> IESIIKTATDTVKSEINAELGVVPSLNAVETGATSNTEPEEAIQTRTVINQHGVSETLVENFLSRAALVSKRSFEYKDHTSSTAQTDKNFFKWTINTRSFVQLRRKLELFTYLRFDAEITILTTVAVNGSNNNTYVGLPDLTLQAMFVPTGALTPEKQDSFHWQSGSNASVFFKISDPPARMTIPFMCINSAYSVFYDGFAGFEKT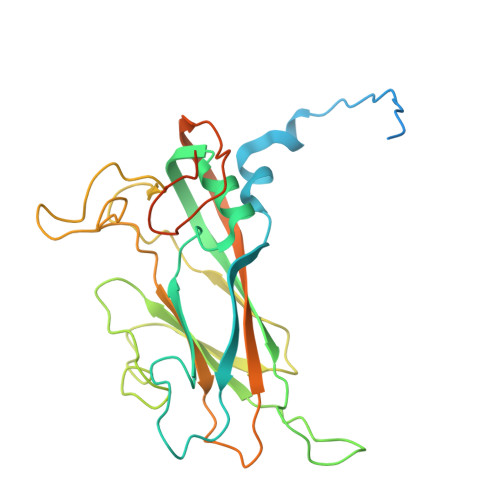GLYGINPADTIGNLCVRIVNEHQPVGFTVTVRVYMKPKHIKAWAPRPPRTLPYMSIANANYKGKERAPNALNAIIGNRDSVKTMPHNIV> SMALSTQLIESVDKQSHLEEQLNKSLKTIASQKAA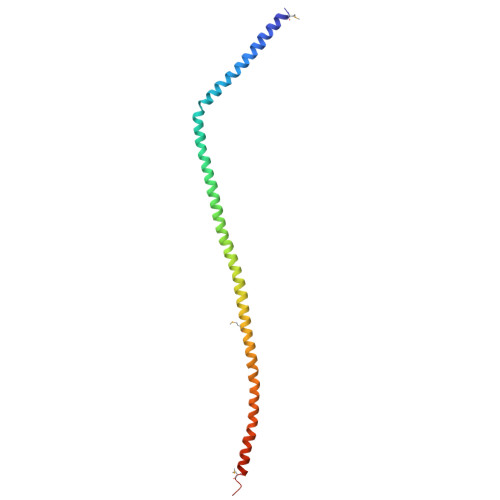IENYNQLKEDYNTLKRELSDRDDEVKRLREDIAKENELRTKAEEEADKLNKEVEDLTASLFDEANNMVADARKEKYAIEILNKRLTEQLREKDTLLDTLTLQLKNLKKVMHSLDNESTV>GPLGSRFNAPQKYQKIKREEFNPETAEKNKIYLLEDQLVYLDIFGKVIDLGQTSDTCHRLFNAITTP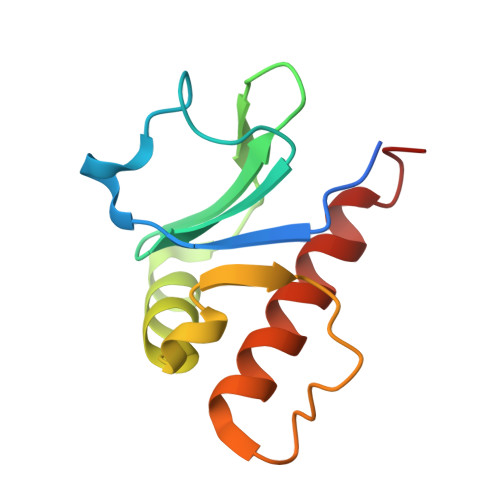FYQNYILYDEYIDPEESAEEAAMFEMGEIVKAKMKNID[2x]>GVFTFEDEITSTVPPAKLYNAMKDADSITPKIIDDVKSVEIVEG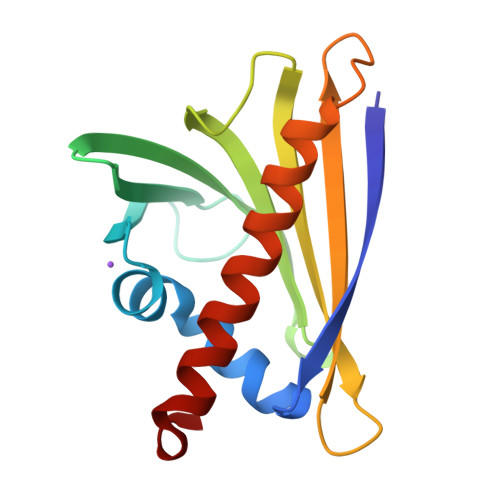NGGPGTIKKLTIVEDGETKFILHKVESIDEANYAYNYSVVGGVALPPTAEKITFETKLVEGPNGGSIGKLTLKYHTKGDAKPDEEELKKGKAKGEGLFRAIEGYVLANPTQY[5x]>MMVAWWSLFLYGLQVAAPALAATPADWRSQSIYFLLTDRFARTDGSTTATCNTADQKYCGGTWQGIIDKLDYIQGMGFTAIWITPVTAQLPQTTAYGDAYHGYWQQDIYSLNENYGTADDLKALSSALHERGMYLMVDVVANHMGYDGAGSSVDYSVFKPFSSQDYFHPFCFIQNYEDQTQVEDCWLGDNTVSLPDLDTTKDVVKNEWYDWVGSLVSNYSIDGLRIDTVKHVQKDFWPGYNKAAGVYCIGEVLDGDPAYTCPYQNVMDGVLNYPIYYPLLNAFKSTSGSMDDLYNMINTVKSDCPDSTLLGTFVENHDNPRFASYTNDIALAKNVAAFIILNDGIPIIYAGQEQHYAGGNDPANREATWLSGYPTDSELYKLIASANAIRNYAISKDTGFVTYKNWPIYKDDTTIAMRKGTDGSQIVTILSNKGASGDSYTLSLSGAGYTAGQQLTEVIGCTTVTVGSDGNVPVPMAGGLPRVLYPTEKLAGSKICSSS[2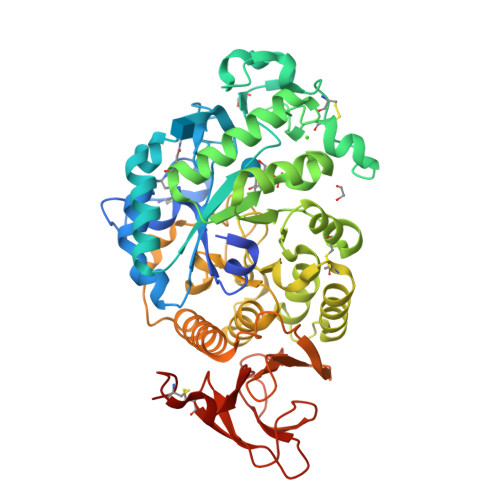x]>MHRYGLLVFCSLVILMVQGVNKAVAGEQAKEVPIPQSISAEFKAALAQYPTPSVEEARSFVPTTAAQWRDYVQATNKMQKTKIKNM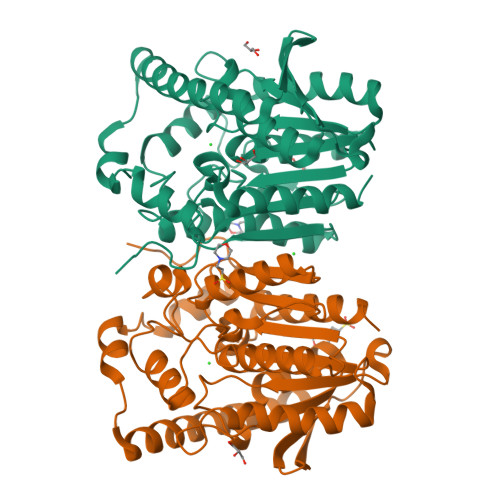RKHYGVTVELLDIKGVTVRKITPKSLSPEFKDHVYIDIHGGAYVLFAGLPSIEEGILIAHRLGIVVYSVDYRMPPAYPFPAALDDVKHVYRVLSQQYDANHIFMGGTSAGGGLLLAFVQGLIENGVATPRAIYAGTPWADLTKTGDSLYTNEGIDRILITYDGTLGASARLYAGNTPLTHPKLSPIYGDFTDFPPTFLVTGTRDMFLSDTVRVNRKMRDAGVTTVLDVYEGLSHADYLVSHQTPESQSVYRQLKRFLVGFTN[8x]Our subsequent work demonstrated that the HEPN protein with a RX4–6H motif is the toxin which cleaves mRNA in vitro in the HEPN/MNT (SO_3166/SO_3165) TA pair in the model psychrotrophic bacterium Shewanella oneidensis. Furthermore, antitoxin SO_3165 binds to toxin SO_3166 at a rare 2:6 ratio to form a hetero-octamer, and this binding is important for the antitoxin to block the toxicity of the toxin. Specifically, structural and biochemical studies of the HepT/MntA TA pair (SO_3166/SO_3165) in S. oneidensis show that the GSX10DXD motif of antitoxin MntA is responsible for transferring three AMPs to HepT and that Y104 in RX4HXY in HepT is the site that receives three AMPs from MntA. We found here that MntA antitoxin acts as an adenylyltransferase and catalyzes the transfer of three AMP moieties onto toxin HepT to block its toxicity, representing a new type of interaction between the toxin and the antitoxin.

To further confirm the role of the conserved MntA GSX10DXD motif in mediating adenylylation, the structure of the HepT/MntAD39E, D41E hetero-octamer was determined at 2.35 Å. The structural analysis confirmed that HepT was not adenylylated even though Y104 was available for receiving AMP. Similarly, substituting the Asp of GSX10DXD with Glu (GSX10EXE) in MntA also eliminated the modification of HepT in the mutated TA complex (HepT/MntAD39E, D41E). The substitutions of DXD with EXE in the GSX10DXD motif also reduced the ability of MntA to neutralize HepT. However, our structural analysis clearly showed that the MntAD39E, D41E variant binds to HepT to form a hetero-octamer in a way that is like native MntA. Additionally, the MntA variants MntAD39E, D41E are still pulled down due to their strong protein-protein interaction with HepT during SDS-PAGE fractionation of the TA complex. These results collectively suggest that the binding to HepT is not sufficient for MntA to neutralize the toxicity of HepT.

>MQQLNENKIIKLLRDNIPKLQLIYLFGSYSQGTQHRNSEIEIAVLAADTLDNIARWELAQKLASALDSDVDLVDLRSASTVLCQQVVTQGKQLWGTQQDDELFAVKTISMYQHLQAERQAIIDDVMANTAAKAHRGESL[2x];>[6x]MNDIIINKIATIKRCIKRIQQVYGDGSQFKQDFTLQDSVILNLQRCCEACIDIANHINRQQQLGIPQSSRDSFTLLAQNNLITQPLSDNLKKMVGLRNIAVHDYQELNLDIVVHVVQHHLEDFEQFIDVIKAE>[4x]AIAMTHPDISVDVLVIGAGPTGLGAAKRLNQIDGPSWMIVDSNETPGGLASTDVTPEGFLYDVGGHVIFSHYKYFDDCLDEALPKEDDWYTHQRISYVRCQGQWVPYPFQNNISMLPKEEQVKCIDGMIDAALEARVANTKPKTFDEWIVRMMGTGIADLFMRPYNFKVWAVPTTKMQCAWLGERVAAPNLKAVTTNVILGKTAGNWGPAATFRFPARGGTGGIWIAVAN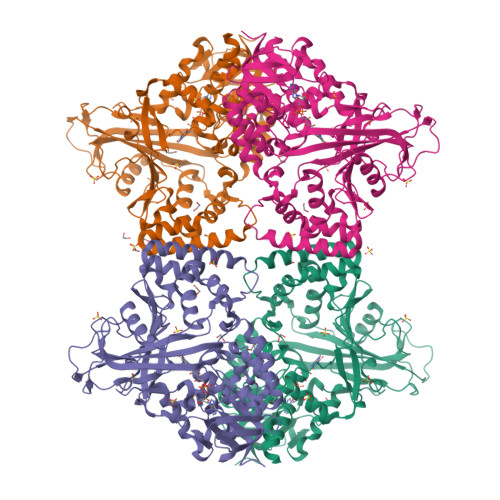TLPKEKTRFGEKGKVTKVNANNKTVTLQDGTTIGYKKLVSTMAVDFLAEAMNDQELVGLTKQLFYSSTHVIGVGVRGSRPERIGDKCWLYFPEDNCPFYRATIFSNYSPYNQPEASAALPTMQLADGSRPQSTEAKEGPYWSIMLEVSESSMKPVNQETILADCIQGLVNTEMLKPTDEIVSTYHRRFDHGYPTPTLEREGTLTQILPKLQDKDIWSRGRFGSWRYEVGNQDHSFMLGVEAVDNIVNGAVELTLNYPDFVNGRQNTERRLVDGAQVFAKSKAQ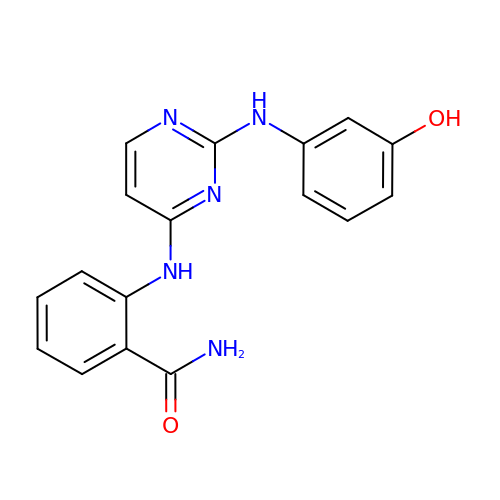2-({2-[(3-HYDROXYPHENYL)AMINO]PYRIMIDIN-4-YL}AMINO)BENZAMIDE | C17 H15 N5 O2 | QHPKKGUGRGRSGA-UHFFFAOYSA-N>[8x]DVYQEPTDPKFPQQWYLSGVTQRDLNVKEAWAQGFTGHGIVVSILD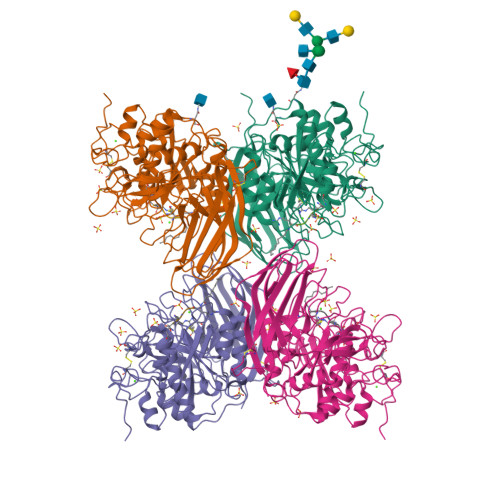DGIEKNHPDLAGNYDPGASFDVNDQDPDPQPRYTQMNDNRHGTRCAGEVAAVANNGVCGVGVAYNARIGGVRMLDGEVTDAVEARSLGLNPNHIHIYSASWGPEDDGKTVDGPARLAEEAFFRGVSQGRGGLGSIFVWASGNGGREHDSCNCDGYTNSIYTLSISSATQFGNVPWYSEACSSTLATTYSSGNQNEKQIVTTDLRQKCTESHTGTSASAPLAAGIIALTLEANKNLTWRDMQHLVVQTSKPAHLNADDWATNGVGRKVSHSYGYGLLDAGAMVALAQNWTTVAPQRKCIVEILVEPKDIGKRLEVRKAVTACLGEPNHITRLEHVQARLTLSYNRRGDLAIHLISPMGTRSTLLAARPHDYSADGFNDWAFMTTHSWDEDPAGEWVLEIENTSEANNYGTLTKFTLVLYGTAPEGL>MNAVEIISRDIYKAIDIQTKILDYMTKFFTDRGFKWLLPIMLSPITDPLWPDPAGEGIRPAEVDVYGVRMRLTHSMILHKQLAIAMGLEKIFVLSPNIRLESRRKDDGRHSYEFTQLDFEIEGAKMKDVMRLIEELIYGLFRKAEEWTGREFPRARHFKVYDYKDILEEFGSDEKASMEMEEPFWIVNIPREFYDREENGVWKNYDLIL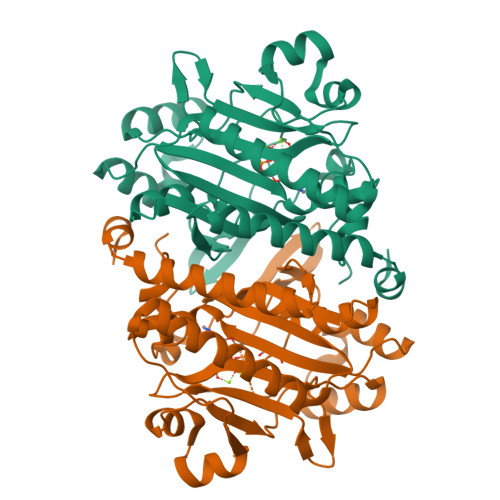PYGYGEVSSGGEREWEYEKIVAKIRAAGLKEDSFRPYLEIARAGKLKPSAGAGIGVERLVRFIVGAKHIAEVQPFPRVPGIPAVI[2x]>SRCTHLENRDFVTGTQGTTRVTLVLELGGCVTITAEGKPSMDVWLDAIYQENPAKTREYCLHAKLSDTKVAARCPTMGPATLAEEHQGGTVCKRDQSDRGWGNHCGLFGKGSIVACVKAACEAKKKATGHVYDANKIVYTVKVEPHTGDYVAANETHSGRKTASFTISSEKTILTMGEYGDVSLLCRVASGVDLAQTVILELDKTVEHLPTAWQVHRDWFNDLALPWKHEGAQNWNNAERLVEFGAPHAVKMDVYNLGDQTGVLLKALAGVPVAHIEGTKYHLKSGHVTCEVGLEKLKMKGLTYTMCDKTKFTWKRAPTDSGHDTVVMEVTFSGTKPCRIPVRAVAHGSPDVNVAMLITPNPTIENNGGGFIEMQL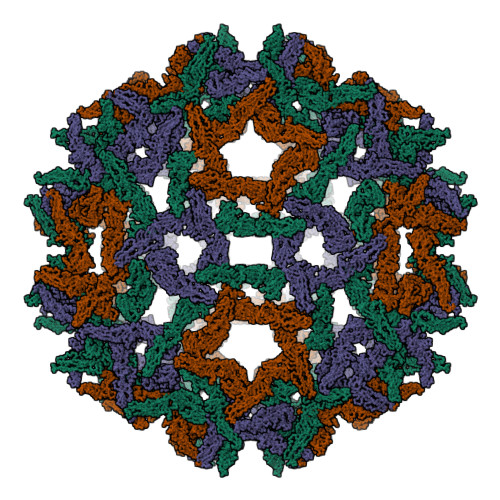PPGDNIIYVGELSHQWFQK[3x]>MRSKRFEALAKRPVNQDGFVKEWIEEGFIAMESPNDPKPSIKIVNGAVTELDGKPVSDFDLIDHFIARYGINLNRAEEVMAMDSVKLANMLCDPNVKRSEIVPLTTAMTPAKIVEVVSHMNVVEMMMAMQKMRARRTPSQQAHVTNVKDNPVQIAADAAEGAWRGFDEQETTVAVARYAPFNAIALLVGSQVGRPGVLTQCSLEEATELKLGMLGHTCYAETISVYGTEPVFTDGDDTPWSKGFLASSYASRGLKMRFTSGSGSEVQMGYAEGKSMLYLEARCIYITKAAGVQGLQNGSVSCIGVPSAVPSGIRAVLAENLICSSLDLECASSNDQTFTHSDMRRTARLLMQFLPGTDFISSGYSAVPNYDNMFAGSNEDAEDFDDYNVIQRDLKVDGGLRPVREEDVIAIRNKAARALQAVFAGMGLPPITDEEVEAATYAHGSKDMPERNIVEDIKFAQEIINKNRNGLEVVKALAQGGFTDVAQDMLNIQKAKLTGDYLHTSAIIVGDGQVLSAVNDVNDYAGPATGYRLQGERWEEIKNIPGALDPNEID[2x];>MEINEKLLRQIIEDVLSEMKGSDKPVSFNAPAASAAPQATPPAGDGFLTEVGEARQGTQQDEVIIAVGPAFGLAQTVNIVGIPHKSILREVIAGIEEEGIKARVIRCFKSSDVAFVAVEGNRLSGSGISIGIQSKGTTVIHQQGLPPLSNLELFPQAPLLTLETYRQIGKNAARYAKRESPQPVPTLNDQMARPKYQAKSAILHIKETKYVVTGKNPQELRVAL[2x];>[2x]MNTDAIESMVRDVLSRMNSLQGEAPAAAPAAGGASRSARVSDYPLANKHPEWVKTATNKTLDDFTLENVLSNKVTAQDMRITPETLRLQASIAKDAGRDRLAMNFERAAELTAVPDDRILEIYNA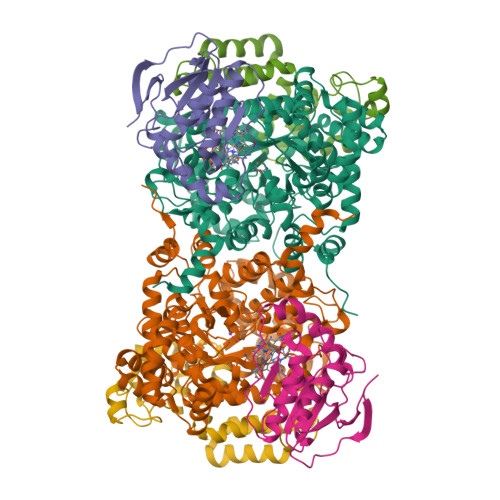LRPYRSTKEELLAIADDLESRYQAKICAAFVREAATLYVERKKLKGDD Isatinic acid | C8 H7 N O3 | 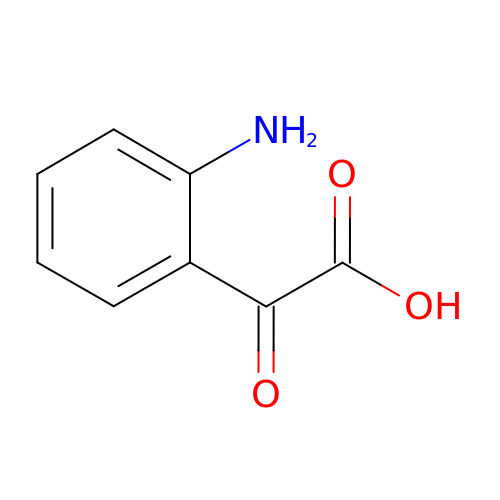MQMWPBBDMIYYMI-UHFFFAOYSA-N>MGD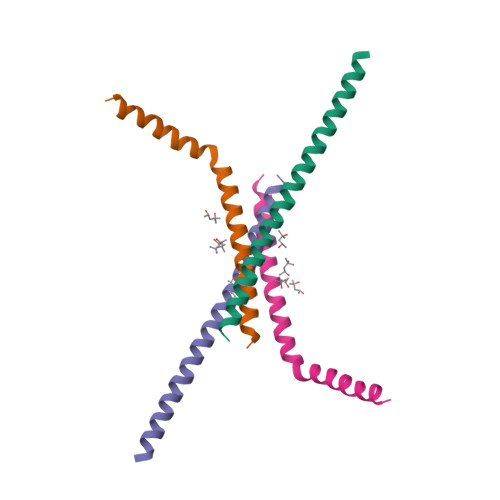QSQKEVWDDSELRNAFETALHEFKKYHSIEAKGYDETYKKLIMSWYYAGYYTGLAEGLAKSEQRKD[2x]> MSYYHHHHHHLESTSLYKKAGSHMDKEGFLNKVREAVDVVKLHIELGHTIRIISHRDADGITSAAILAKALGREGASFHISIVKQVSEDLLRELKDEDYKIFIFSALGSGSLSLIKEYLKEKTVIILDHHPPENVKLEEKHILVNPVQFGANSVRDLSGSGVTYFFARELNEKNRDLAYIAIVGAVGDMQENDGVFHGMNLDIIEDGKSLGILEVKKELRLFGRETRPLYQMLAYATNPEIPEVTGDERKAIEWLKNKGFNPEKKYWELSEEEKKKLHDFLIIHMIKHGAGKEDIDRLIGDVVISPLYPEGDPRHEAREFATLLNATGRLNLGNLGVAVCLGDEEAFRKALKMVEDYKREQIEARKWLLQNWN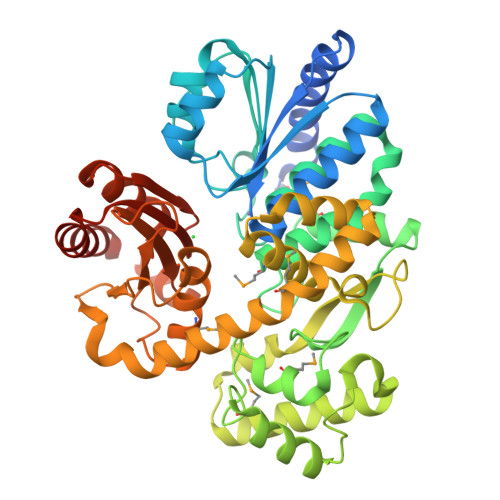SEVWEGDHVYVLYVGKSIRDTLVGIAASMAINAGLADPEKPVIVFADTDEDPNLLKGSARTTERALAKGYNLGEALRKAAELVNGEGGGHAIAAGIRIPRARLAEFRKLIDKILGEQVSKGGDKSES>[2x]MVKETHRFETFTEEPIRLIGEEGEWLGDFPLDLEGEKLRRLYRDMLAARMLDERYTILIRTGKTSFIAPAAGHEAAQVAIAHAIRPGFDWVFPYYRDHGLALALGIPLKELLGQMLATKADPNKGRQMPEHPGSKALNFFTVASPIASHVPPAAGAAISMKLLRTGQVAVCTFGDGATSEGDWYAGINFAAVQGAPAVFIAENNFYAISVDYRHQTHSPTIADKAHAFGIPGYLVDGMDVLASYYVVK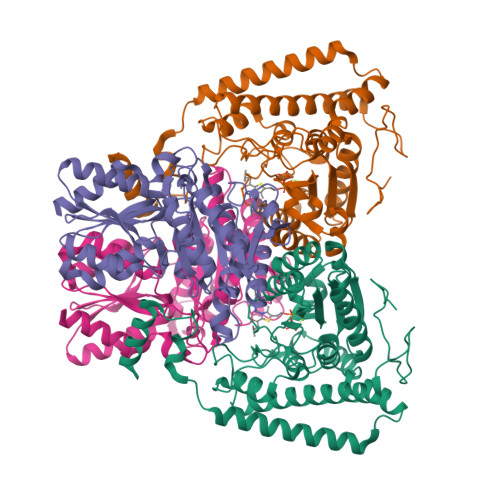EAVERARRGEGPSLVELRVYRYGPHSSADDDSRYRPKEEVAFWRKKDPIPRFRRFLEARGLWNEEWEEDVREEIRAELERGLKEAEEAGPVPPEWMFEDVFAEKPWHLLRQEALLKEEL;>MALMTMVQALNRALDEEMAKDPRVVVLGEDVGKRGGVFLVTEGLLQKYGPDRVMDTPLSEAAIVGAALGMAAHGLRPVAEIQFADYIFPGFDQLVSQVAKLRYRSGGQFTAPLVVRMPSGGGVRGGHHHSQSPEAHFVHTAGLKVVAVSTPYDAKGLLKAAIRDEDPVVFLEPKRLYRSVKEEVPEEDYTLPIGKAALRREGKDLTLICYGTVMPEVLQAAAELAKAGVSAEVLDLRTLMPWDYEAVMNSVAKTGRVVLVSDAPRHASFVSEVAATIAEDLLDMLLAPPIRVTGFDTPYPYAQDKLYLPTVTRILNAAKRALDY[2x]>MGSDKIHHHHHHENLYFQGMYQVVASDLDGTLLSPDHFLTPYAKETLKLLTARGINFVFATGRHYIDVGQIRDNLGIRSYMITSNGARVHDSDGQQIFAHNLDRDIAADLFEIVRNDPKIVTNVYREDEWYMNRHRPEEMRFFKEAVFNYKLYEPGELDPQGISKVFFTCEDHEHLLPLEQAMNARWGDRVNVSFSTLTCLEVMAGGVSKGHALEAVAKMLGYTL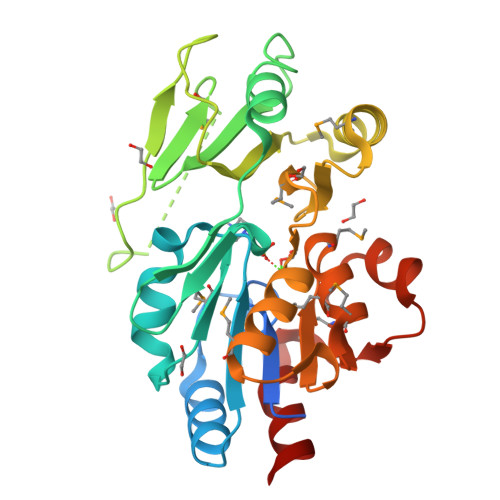SDCIAFGDGMNDAEMLSMAGKGCIMANAHQRLKDLHPELEVIGSNADDAVPRYLRKLYLD[4x]> AEFGSHHHHHHGSAPMAEGGGQNHHEV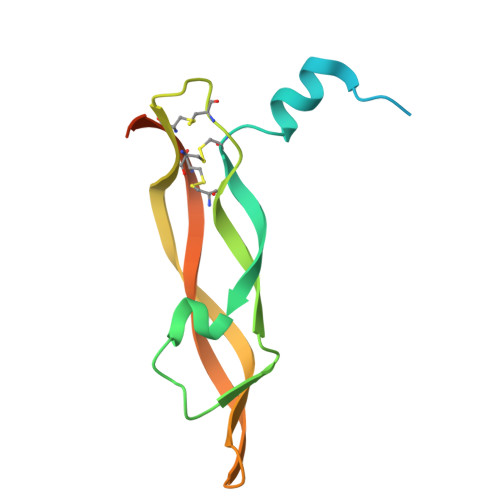VKFMDVYQRSYCHPIETLVDIFQEYPDEIEYIFKPSCVPLMRCGGCCNDEGLECVPTEESNITMQIMRIKPHQGQHIGEMSFLQHNKCECRPKKDRARQENCDKPRR In this work, the structural and functional characterization of PnpA, an NlpC/P60 family peptidase secreted by Photobacterium damselae subsp. piscicida (Phdp) is reported. The results show that PnpA is a PG hydrolase with a four-domain structure similar to that of Desulfovibrio vulgaris lysin (DvLysin) and specificity for the γ-d-glutamyl-meso-diaminopimelic acid bond, but with a more hydrophobic and narrower access to the catalytic center. It is also shown that PnpA is secreted into the extracellular medium by the Phdp type II secretion system and acts on the PG of Vibrio anguillarum and Vibrio vulnificus, suggesting that it may provide Phdp an advantage over bacteria competing for the same resources or a way of obtaining nutrients in nutrient-scarce environments, either inside or outside the host. PnpA is not essential for Phdp cell wall biogenesis and does not cleave Phdp PG, but it degrades the PG of V. anguillarum and V. vulnificus, two bacterial species that share the same hosts and/or environment as Phdp.

The crystal asymmetric unit contains two PnpA molecules, which are essentially identical (root mean square deviation [RMSD], of 0.5 Å for 457 aligned Cα atoms). Analysis of the intermolecular packing interfaces within the crystal lattice suggests that the molecule behaves as a monomer in solution, which is in agreement with the molecular mass estimated by size exclusion chromatography. The PnpA monomer has an overall structure similar to that of DvLysin, namely, one N-terminal “c-clip” or “N_NLPC_P60” stabilizing domain (residues N20-N133), two SH3b domains (SH3b1, residues I134-V218; SH3b2, residues D219-T295), and the C-terminal NlpC/P60 catalytic domain (residues P296-K499). As in DvLysin, the PnpA c-clip domain has an extended helical conformation which surrounds and stabilizes the SH3b1 and NlpC/P60 domains, forming a planar assembly from which the SH3b2 domain protrudes. Compared to DvLysin, the c-clip domain of PnpA harbors an extension between helices α1 and α2, thereby forming an additional two-stranded antiparallel β-sheet (β2 and β3) and a 310 helix (η4), which protrude into the catalytic groove and close one of its sides. While this topology is generally maintained in PnpA, the end of the groove opposite to the RT loop is also closed by strands β2 and β3 and the 310 helix η4, creating a narrower access to the catalytic site. In PnpA, the residues that make up the active site are C324, H395, and N415, the latter similar to the equivalent residue found in the active site of the prototypical papain, but differing from the histidine (H408) at the active site of DvLysin. In the PnpA structure, the thiol group of the catalytic cysteine is oxidized, resulting in the disruption of the characteristic C324 SD-H395 ND1 hydrogen bond and suggesting that the enzyme is in an inactive state.

>MNINKHLMLLALLTNYSYANGNNITIPIEITQDAFHYISHKDLDKNIIDKYTIRQMNEYFNTQYYFQWSDDANQNDFYYVPNNTQTKNNILKLENDTIRYYKERSGYDKNYLPHTSNWVNSISENMNLKSFPNIPCDNHSCRGIVVNNAQVRSLPTSDAFYNNFTIPGEGYPFDYIQLSALWTGTPIMLIHMSTDKKWTLIKGQGTLGWVPTSSIANVDESFITQWKRYRLVTPTVRKQDLPIEKYDINNKILEAGSILPEHKGKLKIPVKDKNGTATLLTVNSKNLKFTTWPMTPSYKNFAHQINNYIGMPYGWGGMDFNNDCSGLLKRLFSTFGIWLPRSSFYQANYAGQIYSMYDQSEEQRKELLVEQEGSIQLIPFMTLVSFGNSKTSTSHIGLYMGTTEYNHNKVAIMFNAPWGVKLVNGNNEQGRALVGQTLITPIGIGDAFTEGLSNQDWALQSLWNAVGFNTTLLTETPKNKRLYQGIDNSYSIEKYLFEK[2x]>PNIEMFVVEGYSDQQKEALVGALTQATVEAIGAPIDSVRVWLTEVPATQFGIGGKTVAAIAAGQESAADGAPPSLSIIQVTFIAGRTELQKERLIAALTDAAVDTVGIERAEVRVILKDIPNTDYGIAGQTARSLGRGVDRHGRAPG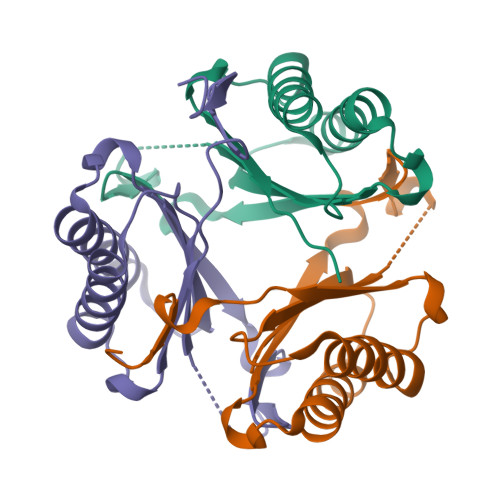GS[3x]>[8x]GLDNELSLVDGQDRTLTVQQWDTFLNGVFPLDRNRLTREWFHSGRAKYIVAGPGADEFEGT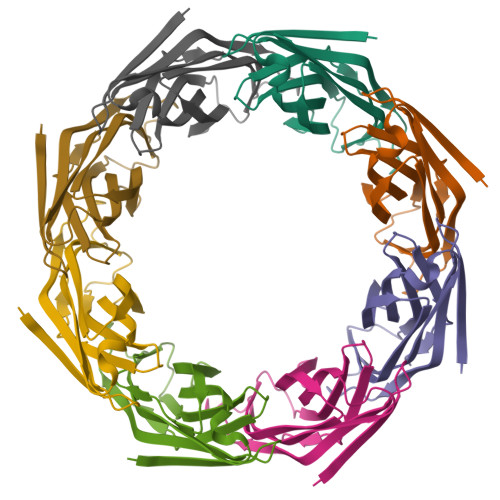LELGYQIGGPGIQEVATFSVDVSGAEGGVAVSNAHGTVTGAAGGVLLRPFARLIASTGDSVTTYGEPWNMN> GTEAVGHFEGRSVTRAAVRGEDRSSVAGLARWLARNVAGDPRSEQALQRLADGDGTPLEARTVR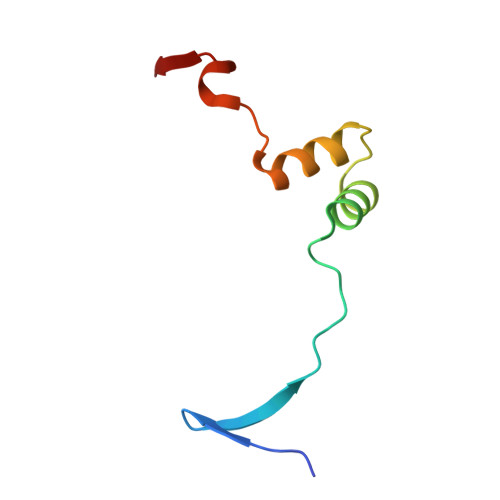RR>MTLNTIALQLVPPNSDGPDGGREQAVEDARKVLRCAAETGLAGRIGHVMIPGMIEEDPDRPIPMKPKMDVLDFWTIIRPELPGIRGLCTQVTAFLDEPALRRRLGDLSAAGFDGIAFVGVPRTMNDGEGHGVAPTDALSMFADLVPNRGAILIPTRDGEQGRFEFKCERGATYGMTQLLYSDAIVGFLREFARRTDHRPEILLSFGFVPKLEAKVGLINWLIQDPGNPAVAAEQEFVRRLAGLEPADKRKLMVDLYKRVIDGVADLGFPLSVHLEATYGVSVPAFETFAE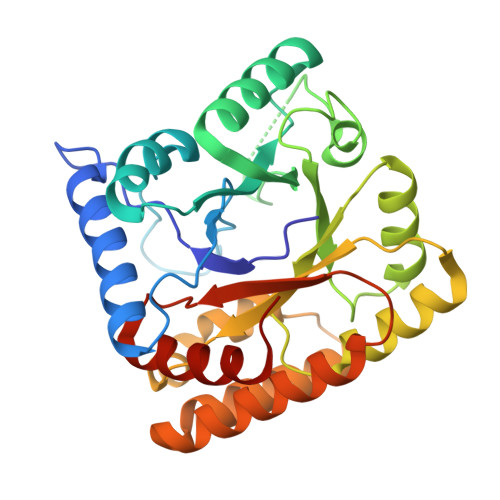MLAYWSPGQG[2x]Of the receptors known to regulate CYP3A4 transcription, PXR is the main ligand-dependent CYP3A4 regulator and is renowned for its highly promiscuous ligand binding pocket. Here, we show that JQ1 and the BET-inactive (−)-JQ1 are agonists of pregnane X receptor (PXR), a nuclear receptor that transcriptionally regulates genes encoding drug-metabolizing enzymes such as CYP3A4, which was previously shown to oxidize JQ1. To differentiate between PXR activation and BET inhibition, we show that JQ1 binds directly to the PXR ligand binding domain (LBD), induces recruitment of transcriptional coactivator to PXR, exhibits selectivity for human PXR over mouse PXR (mPXR), and can be blocked by a PXR antagonist. Because a PXR agonist is expected to induce recruitment of transcriptional coactivators (i.e. SRC-1), we assessed interaction of purified PXR LBD with a 23 amino acid SRC-1 peptide and found that JQ1 induced SRC-1 recruitment.

To investigate the binding mode of JQ1 to PXR LBD, we solved the PXR LBD-JQ1 co-crystal structure in the presence of coactivator SRC-1 peptide. Consistent with previously reported structures, the asymmetric unit contained two PXR LBD (chains A and B) and two SRC-1 peptides (chains C and D). In both PXR LBD chains, the thienotriazolodiazepine core and tert-butyl acetate group of JQ1 were clearly resolved, but weaker density was observed for the chlorophenyl appendage. While the tert-butyl group was anchored in an aromatic cage made up of F288, W299, and Y306 that has been shown to trap a large proportion of PXR ligands, the chlorophenyl was positioned near a void and oriented toward alpha helix 2 (α2), which is highly flexible and not observed in certain previous structures. Interestingly, α2 was present in chain A but was not resolved in chain B, indicating that the close proximity of the chlorophenyl to the region displaces or destabilizes α2. When residues within 5 Å of JQ1 in chain A were analyzed, we observed a void between α2 (S208 and L209) and α3 (L240, M243, and A244) that may allow the chlorophenyl and additional groups to freely move. Indeed, JQ1 clearly has at least two binding poses since two different modes were observed between the two PXR LBD chains. This plasticity and differential positioning of the tert-butyl acetate moiety illustrate how binding by (−)-JQ1 is possible, as there is sufficient space for either enantiomer to bind. The flexibility observed in the PXR LBD-JQ1 co-crystal structure contrasts with the constrained binding poses in bromodomain-JQ1 structures, highlighting the structural features that allow PXR to bind diverse molecules.

>MGKGHHHHHHGSERTGTQPLGVQGLTEEQRMMIRELMDAQMKTFDTTFSHFKNFRLPGVLSSGCELPESLQAPSREEAAKWSQVRKDLCSLKVSLQLRGEDGSVWNYKPPADSGGKEIFSLLPHMADMSTYMFKGIISFAKVISYFRDLPIEDQISLLKGAAFELCQLRFNTVFNAETGTWECGRLSYCLEDTAGGFQQLLLEPMLKFHYMLKKLQLHEEEYVLMQAISLFSPDRPGVLQHRVVDQLQEQFAITLKSYIECNRPQPAHRFLFLKIMAMLTELRSINAQHTQRLLRIQDIHPFATPLMQELFGITGS[2x];>[2x]CPSSHSSLTERHKILHRLLQEGSPS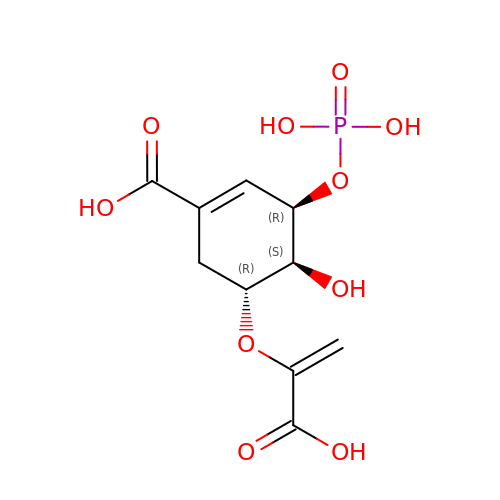5-[(1-CARBOXYVINYL)OXY]-4-HYDROXY-3-(PHOSPHONOOXY)CYCLOHEX-1-ENE-1-CARBOXYLIC ACID | C10 H13 O10 P | QUTYKIXIUDQOLK-PRJMDXOYSA-N> MGHHHHHHGRAMNNPAIKRIGNHITKSPEDKREYRGLELANGIKVLLISDPTTDKSSAALDVHIGSLSDPPNIAGLSHFLQHMLFLGTKKYPKENEYSQFLSEHAGSSNAFTSGEHTNYYFDVSHEHLEGALDRFAQFFLSPLFDESAKDREVNAVDSEHEKNVMNDAWRLFQLEKATGNPKHPFSKFGTGNKYTLETRPNQEGIDVRQELLKFHSAYYSSNLMAVVVLGRESLDDLTNLVVKLFSEVENKNVPLPEFPEHPFQEEHLKQLYKIVPIKDIRNLYVTFPIPDLQKYYKSNPGHYLGHLIGHEGPGSLLSELKSKGWVNTLVGGQKEGARGFMFFIINVDLTEEGLLHVEDIILHMFQYIQKLRAEGPQEWVFQELKDLNAVAFRFKDKERPRGYTSKIAGILHYYPLEEVLTAEYLLEEFRPDLIEMVLDKLRPENVRVAIVSKSFEGKTDRTEEWYGTQYKQEAIPDEVIKKWQNADLNGKFKLPTKNEFIPTNFEILPLEKEATPYPALIKDTAMSKLWFKQDDKFFLPKANLNFEFFSPFAYVDPLHSNMAYLYLELLKDSLNEYAYAAELAGLSYDLQNTIYGMYLSVKGYNDKQPILLKKIIEKMATFEIDEKRFEIIKEAYMRSLNNFRAEQPHQ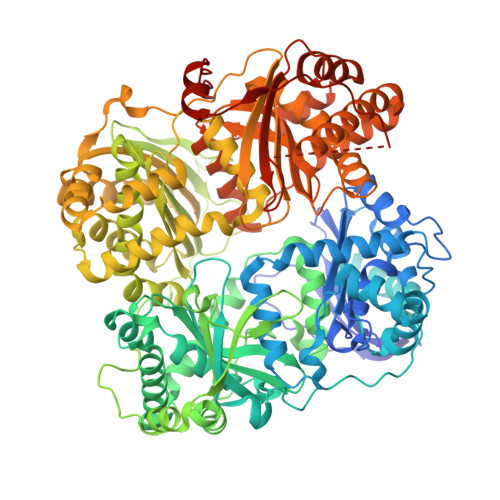HAMYYLRLLMTEVAWTKDELKEALDDVTLPRLKAFIPQLLSRLHIEALLHGNITKQAALGIMQMVEDTLIEHAHTKPLLPSQLVRYREVQLPDRGWFVYQQRNEVHNNSGIEIYYQTDMQSTSENMFLELFAQIISEPAFNTLRTKEQLGYIVFSGPRRANGIQGLRFIIQSEKPPHYLESRVEAFLITMEKSIEDMTEEAFQKHIQALAIRRLDKPKKLSAESAKYWGEIISQQYNFDRDNTEVAYLKTLTKEDIIKFYKEMLAVDAPRRHKVSVHVLAREMDSNPVVGEFPAQNDINLSQAPALPQPEVIQNMTEFKRGLPLFPLVKPHINFMAAKL> MGSSHHHHHHSSGLVPRGSMRGSHMPEGTLQLWTLQLAPKFNPYMDDVLGSWDKLHPEALVRWTDLPWGSVERKLLAAVFARTAPDVVNLNPPFAANLASKGGLTDLTALLPPGAEQNYLPSVWEAARDPEAGQIA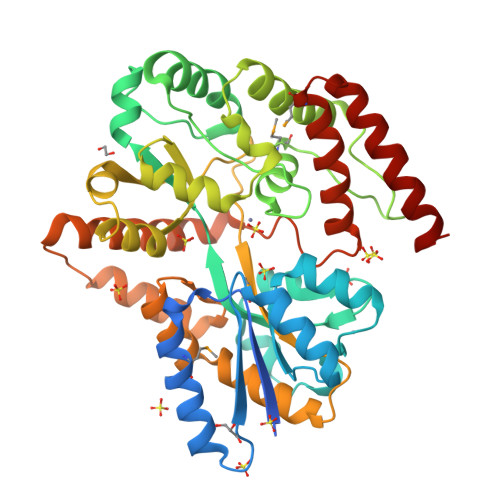IPWYLTVRLSLVNGDLLRQAGLSRAPRRWDEVPAYARSIRERTGRYGLFVTVVPDDSAELLESFVQMGVSLLDARQRAAFNTPAGRKAFAFWTDLYREGLLPREVVSQGQRRAIELYQSGELALLASGAEFLRSIQTNAPGVAAVTTPQPPLTGSDGTANVALMTLAVPRQSQQAGEAVELALFLTNGTNQARFAREARVLPSSLEALSAIRAELEVEQPSNPAEAQIRDARLLSAETLNTARVLVPATPGVKRLQSIIYTQLQRAMLGQISSDQAVLEAEQQWNRYASARWP>GAMGKVTHSIHIEKSDTAADTYGFSLSSVEEDGIRRLYVNSVKETGLASKKGLKAGDEILEINNRAADALNSSMMED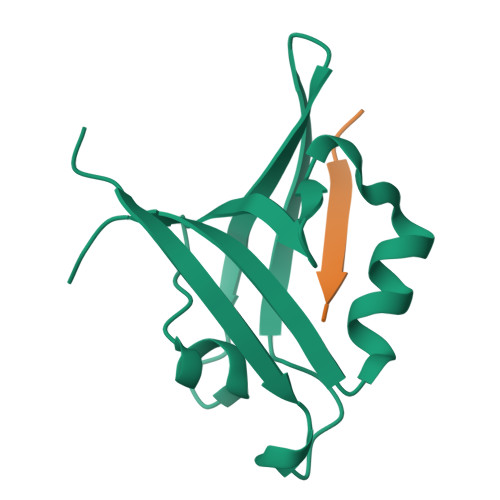FFSQPSVGLLVRTYPEL[3x];>ENQKEYFF[3x]> SVVVQLTMAFREGTINVHDVETQFNQYKTEAASRYNLTISDVSVSDVPFPF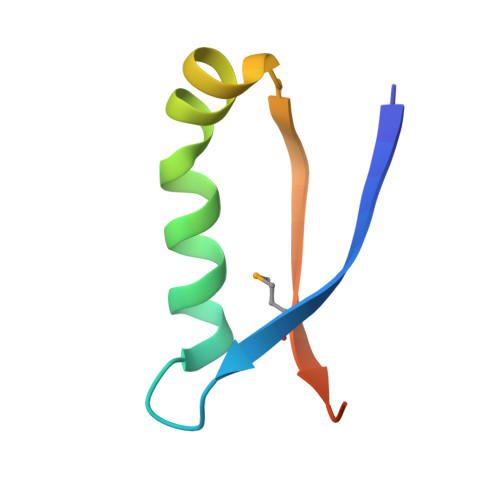SAQS> MAFNDLLQQVGGVGRFQQIQVTLVVLPLLLMASHNTLQNFTAAIPTHHCRPPADANLSKNGGLEVWLPRDRQGQPESCLRFTSPQWGLPFLNGTEANGTGATEPCTDGWIYDNSTFPSTIVTEWDLVCSHRALRQLAQSLYMVGVLLGAMVFGYLADRLGRRKVLILNYLQTAVSGTCAAFAPNFPIYCAFRLLSGMALAGISLNCMTLNVEWMPIHTRACVGTLIGYVYSLGQFLLAGVAYAVPHWRHLQLLVSAPFFAFFIYSWFFIESARWHSSSGRLDLTLRALQRVARINGKREEGAKLSMEVLRASLQKELTMGKGQASAMELLRCPTLRHLFLCLSMLWFATSFAYYGLVMD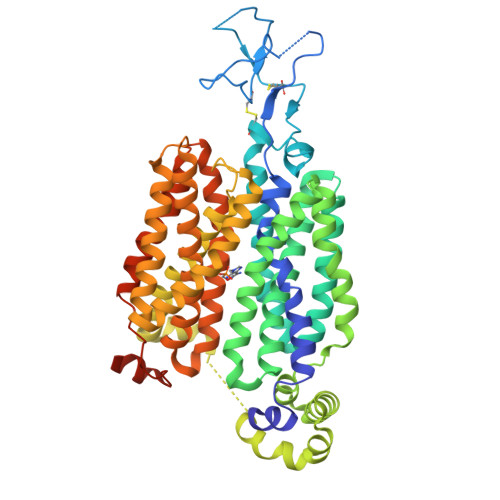LQGFGVSIYLIQVIFGAVDLPAKLVGFLVINSLGRRPAQMAALLLAGICILLNGVIPQDQSIVRTSLAVLGKGCLAASFNCIFLYTGELYPTMIRQTGMGMGSTMARVGSIVSPLVSMTAELYPSMPLFIYGAVPVAASAVTVLLPETLGQPLPDTVQDLESRHHHHHHHHHHGSVEDYKDDDDK4-{3-chloro-5-[(E)-2-cyanoethenyl]phenoxy}-3-[2-(2,4-dioxo-3,4-dihydropyrimidin-1(2H)-yl)ethoxy]phenyl 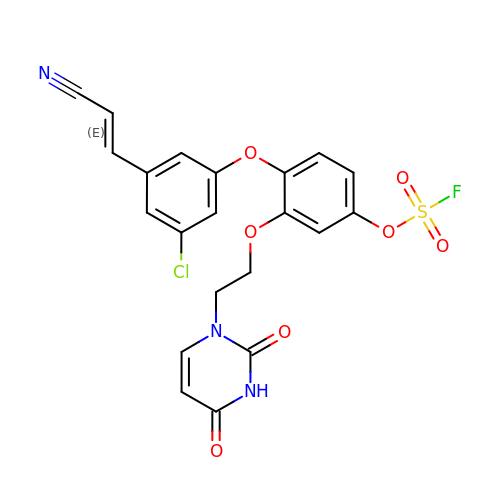sulfurofluoridate | C21 H15 Cl F N3 O7 S | RUPMZEQONCTYBJ-OWOJBTEDSA-N> GPMGVVEEAHNVKVIGSGEATIVLGHGFGTDQSVWKHLVPHLVDDYRVVLYDNMGAGTTNPDYFDFDRYSNLEGYSFDLIAILEDLKIESCIFVGHSVSAMIGVLASLNRPDLFSKIVMISASPRYVNDVDYQGGFEQEDLNQLFEAIRSNYKAWCLGFAPLAVGGDMDSIAVQEFSRTLFNMRPDIALSVGQTIFQSDMRQILPFVTVPCHILQSVKDLAVPVVVSEYLHANLGCESVVEVIPSDGHLPQLSSPDSVIPVILRHIR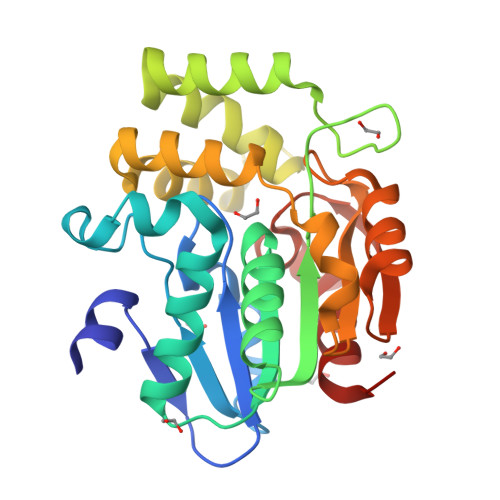NDIAM> HIDPESKIKDCPWYDRGFCKHGPLCRHRHTRRVICVNYLVGFCPEGPSCKFMHPRFE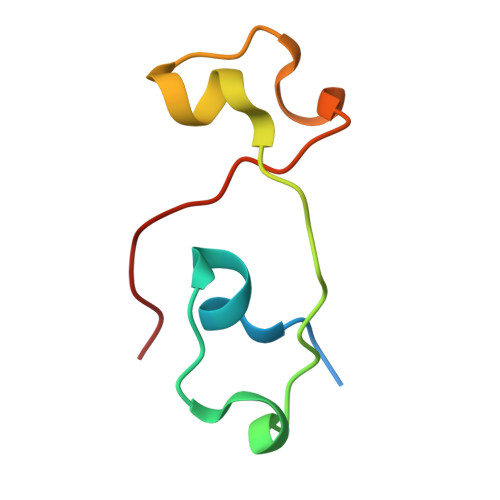LPM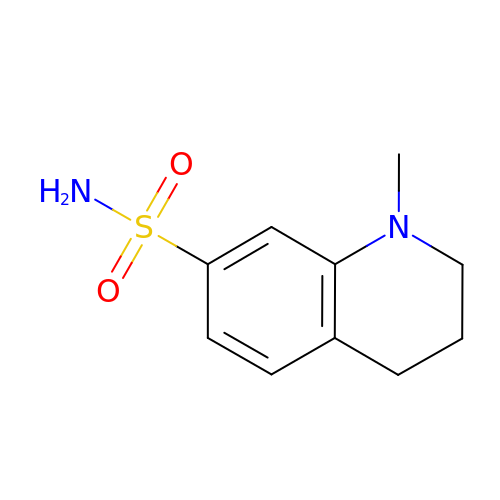1-methyl-3,4-dihydro-2~{H}-quinoline-7-sulfonamide | C10 H14 N2 O2 S | OUJFDUTZTPBMDN-UHFFFAOYSA-N> GGSAPIPDLKVFEREGVQLNLSFIRPPENPALLLITITATNFSEGDVTHFICQAAVPKSLQLQLQAPSGNTVPARGGLPITQLFRILNPNKAPLRLKLRLTYDHFHQSVQEIFEVNNLPVESWQ;> GEEWG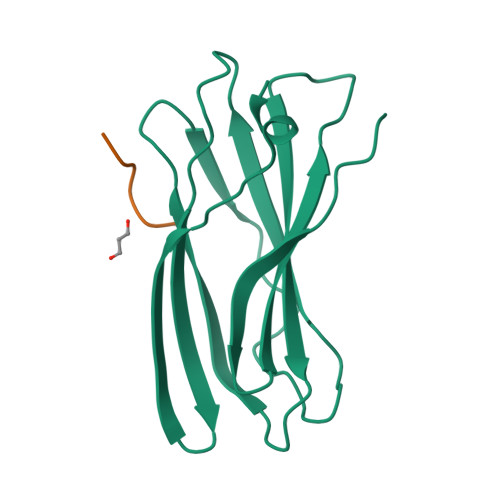PWVX>[2x]HHHHHHSSGLVPRGSHMAIATINPTTGEICQRFKALTPAEIDAKLAKAQEAFQAYRRTSFSQRRQWLENAAAILERDTSKFAEIMTTEMGKTHQSAIAE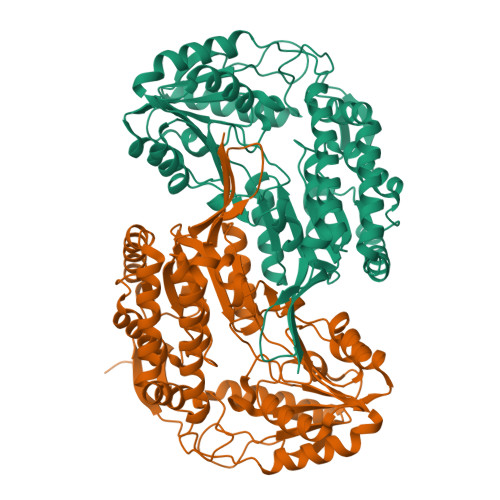AEKSALVCRYYAEHGEQFLANEYTETQATESYVCYQPLGILLAVMPWNFPFWQVFRFAAPALMAGNVAVLKHASNVPQCALAVEAILEAAGFPEGVFQTLLIGASQVEQVIKDPRVKAATLTGSEPAGASLASLAGQEIKPTLLELGGSDPFVVFPSADLDEAVEVGTVARTMNNGQSCIAAKRFILHEAIAAEFLEKLHLKFASLKIGDPMAPETDIGPLATEGILQDISRQVDQAVAAGAKILLGGRPLDRAGYFYPPTILTEIPPGAKILQEELFAPVAMVFTVKDLDQAIALANDIPFGLGASAWTNDPAEQQRFIQELDAGAVFINGMVKADPRLPFGGTKRSGYGRELGLAGIRTFVNAKTVWLK Glutathione transferases (GSTs) are promiscuous enzymes whose main function is the detoxification of electrophilic compounds. The isoenzyme hGSTA1-1 is primarily expressed in the human liver but can also be found in various other human tissues. It is a key enzyme in human physiology, since it is involved in the phase II detoxification mechanism of a wide range of electrophilic compounds, such as drugs, carcinogenic metabolites, and environmental pollutants. Cytosolic GSTs are dimeric enzymes with each subunit having two distinct domains: a conserved N-terminal thioredoxin-like α/β domain and a C-terminal α-helical domain.

The improvement in the catalytic activity of hGSTA1-K141H/S142H as well as its thermal stability prompt us to investigate the structure of this mutant at the atomic level using X-ray crystallography. The mutant was crystallized in two crystal forms with four molecules (1.56 Å resolution) and two molecules (1.87 Å), respectively, in the crystallographic asymmetric unit. Both forms display the typical dimer state found in other GSTs. Residues 212–221 at the C-terminal were not included in the structure because of high disorder. The analysis revealed that each monomer of hGSTA1-K141H/S142H retains the well-established structural features of GSTs, which consist of the presence of two distinct domains. The engineered amino acids are at the surface of the enzyme. The results showed that the mutant hGSTA1-K141H/S142H exhibits higher catalytic efficiency, thermal stability, and sensitivity against α-endosulfan compared to the wild-type enzyme. The double mutation K141H/S142H, according to the crystallographic analysis, results in subtle but specific changes in the protein structure, and the observed stability may be attributed to specific interactions within an amino acid network. The results demonstrate that the mutant hGSTA1-K141H/S142H depicts higher catalytic efficiency and stability than the rest of the mutants studied; the mutation S142H is likely the main contributor. The enhanced stability properties of hGSTA1-K141H/S142H, along with its increased catalytic activity, can make this hGSTA1-1 variant a new potential scaffold for future applications.

>[2x]MAEKPKLHYFNARGRMESTRWLLAAAGVEFEEKFIKSAEDLDKLRNDGYLMFQQVPMVEIDGMKLVQTRAILNYIASKYNLYGKDIKERALIDMYIEGIADLGEMILLLPVCPPEEKDAKLALIKEKIKNRYFPAFEKVLHHHGQDYLVGNKLSRADIHLVELLYYVEELDSSLISSFPLLKALKTRISNLPTVKKFLQPGSPRKPPMDEKSLEEARKIFRF>[4x]MTRYQNLVNGKWKSSEQEITIYSPINQEELGTVPAMTQ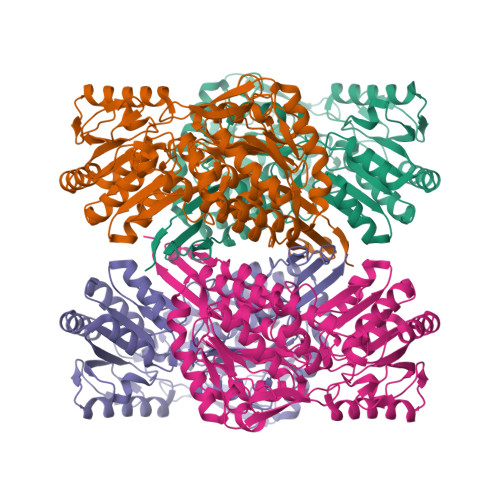TEADEAMQAARAALPAWRALSAIERAAYLHKTAAILERDKEKIGTILAKEVAKGIKAAIGEVVRTADLIRYAAEEGLRITGQAMEGGGFEAASKNKLAVVRREPVGIVLAIAPFNYPVNLSASKIAPALIAGNVVMLKPPTQGSISGLLLAKAFEEAGIPAGVFNTITGRGSEIGDYIIEHKEVNFINFTGSTPIGERIGRLAGMRPIMLELGGKDAALVLEDADLEHAAKQIVAGAFSYSGQRCTAIKRVIVLESVADKLATLLQEEVSKLTVGDPFDNADITPVIDNASADFIWGLIEDAQEKEAQALTPIKREGNLLWPVLFDQVTKDMKVAWEEPFGPVLPIIRVASVEEAIAFANESEFGLQSSVFTNDFKKAFEIAEKLEVGTVHINNKTQRGPDNFPFLGVKGSGAGVQGIKYSIEAMTNVKSIVFDVK> AELISKEGNKVEFKVSVPAAEVNRAYDQVWAGLARDVRVPGFRPGKAPRKVIENRVGKGYVESQVRDRLLETHYSQGLRELG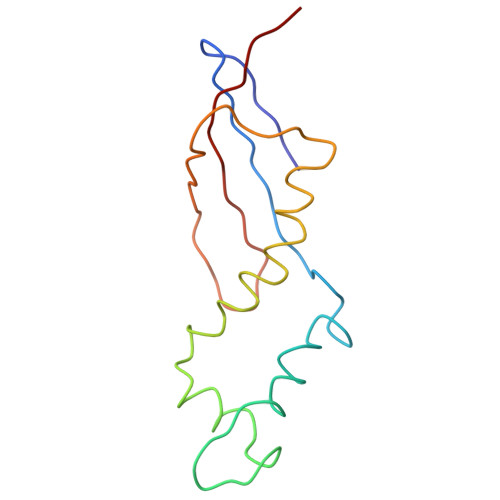LNLVDATVDPQDVQSGQAFEFTVKGETYPEV> MDALSNGIKKHRTSLPSPMFSRNDFSIWSILRKCIGMELSKITMPVIFNEPLSFLQRLTEYMEHTYLIHKASSLSDPVERMQCVAAFAVSAVASQWERTGKPFNPLLGETYELVRDDLGFRLISEQVSHHPPISAFHAEGLNNDFIFHGSIYPKLKFWGKSVEAEPKGTITLELLEHNEAYTWTNPTCCVHNIIVGKLWIEQYGNVEIINHK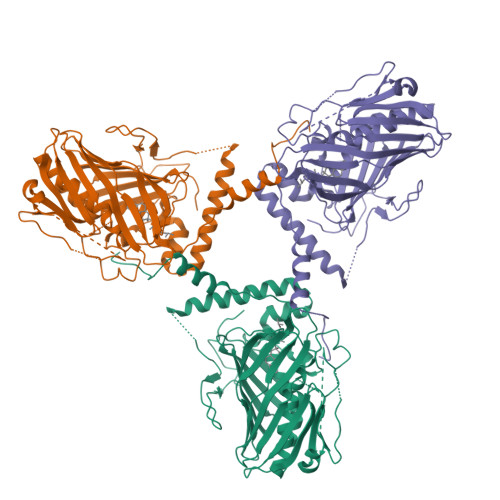TGDKCVLNFKPCGLFGKELHKVEGYIQDKSKKKLCALYGKWTECLYSVDPATFDAYKKNDKKNTEEKKNSKQMSTSEELDEMPVPDSESVFIIPGSVLLWRIAPRPPNSAQMYNFTSFAMVLNEVDKDMESVIPKTDCRLRPDIRAMENGEIDQASEEKKRLEEKQRAARKNRSKSEEDWKTRWFHQGPNPYNGAQDWIYSGSYWDRNYFNLPDIYLEHHHHHH> ALPQTVRIGTDTTYAPFSSKDAKGEFIGFDIDLGN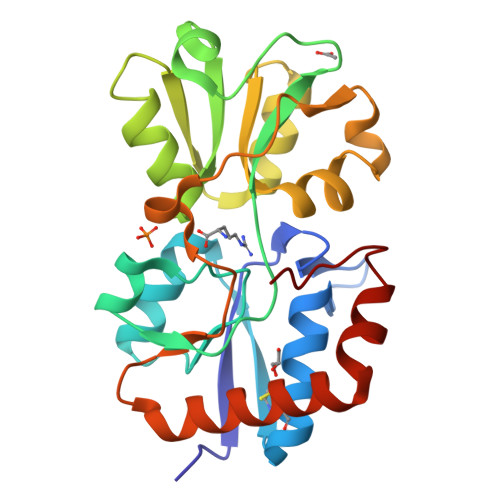EMCKRMQVKCTWVASDFDALIPSLKAKKIDAIISSLSITDKRQQEIAFSDKLYAADSRLIAAKGSPIQPTLESLKGKHVGVLQGSTQEAYANDNWRTKGVDVVAYANQDLIYSDLTAGRLDAALQAEVAASEGFLKQPAGKEYAFAGPSVKDKKYFGDGTGVGLRKDDTELKAAFDKALTELRQDGTYDKMAKKYFDFNVYGD>SNAGGSATGTGLVYVDAFTRFHCLWDASHPECPARVSTVMEMLETEGLLGRCVQVEARAVTEDELLLVHTKEYVELMKSTQNMTEEELKTLAEKYDSVYLHPGFFSSACLSVGSVLQLVDKVMTSQLRNGFSINRPPGHHAQADKMNGFCMFNNLAIAARYAQKRHRVQRVLIVDWDVHHGQGIQYIFEEDPSVLYFSVHRYEDGSFWPHLKESDSSSVGSGAGQGYNINLPWNKVGMESGDYITAFQQLLLPVAYEFQPQLVLVAAGFDAVIGDPLGGMQVSPECFSILTHMLKGVAQGRLVLALEGGYNLQSTAEGVCASMRSLLGDPCPHLPSSGAPCESALKSISKTISDLYPFWK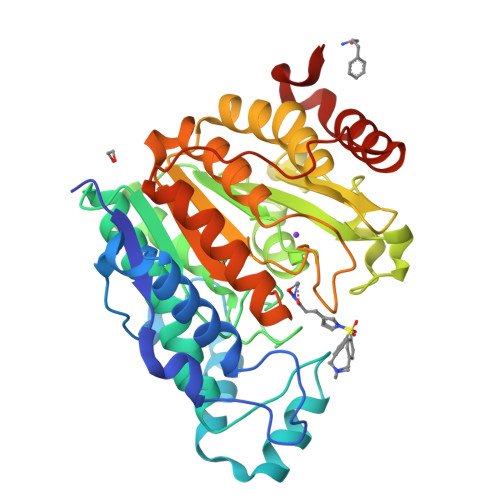SLQTFE[2x]> GSHMESGDEAAIERHRVHLRSATLRDAVPATLHLLPCEVAVDGPAPVGRFFTPAIRQGPEGLEVSFRGRCLRGEEVAVPPGLVGYVMVTEEKKVSMGKPDPLRDSGTDDQEEEPLERDFDRFIGATANFSRFTLWGL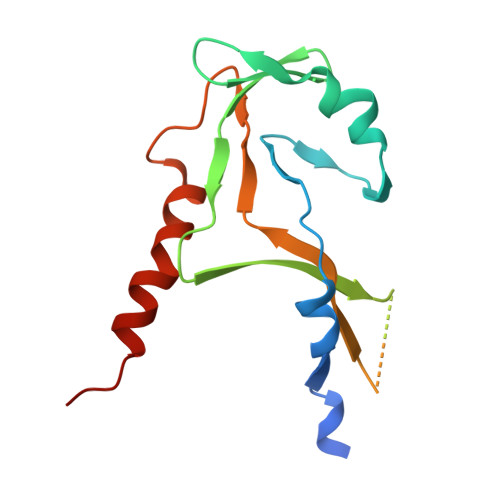ETIPGPDAKVRGALTWPSLAAAIHAQVPED>MAHHHHHHMSMFNIVRKEFQFGQHQVVLETGRVARQANTVLITMGGVTVLVAVVAAPTAKAGQDFFPLTVNYQEKQYAAGRIPGGYGKREGRASEAETLISRLIDRPIRPLFPEGYYNEIQVTATVVSSDKTMEADIAAMLGTSAALAIAGTPFRGPIGAARVGLINGEYVLNPNFEQMAQSDLDLVVAGTESAVLMVESEAKELSEDQMLGAVLFGHDEMQIAIQAINEFAAAAGAKPSDWVAPAHNEELRAKLKEAFEAKISEAYTIAVKQDRYAALDALHAEAVAQFVPEEDVDGIADEVDYLFEDLKYRTVRDNILSGKPRIDGRDTKTVRALDVQVGVLERAHGSALFTRGETQALVTTTLGNTRDALMVDTLAGTKTDNFMLHYNFPAYSVGETGRE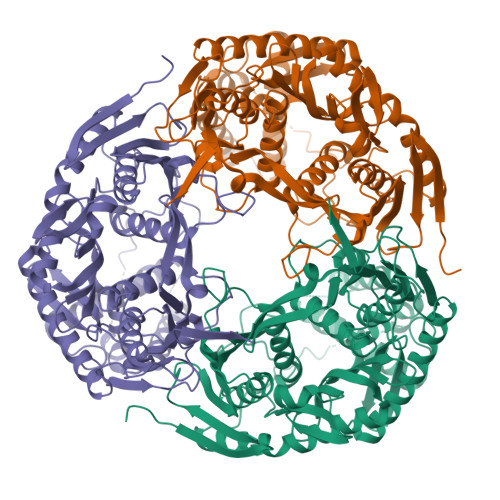SGPKRREIGHGRLARRGVQAVLPAADRFPYVIRIVSDITESNGSSSMASVCGASLSLMDAGVPLKAPVAGIAMGLVKEGERFAVLSDILGDEDHLGDMDFKVAGSANGITALQMDIKIEGITEEIMEVALNQAFAGRMHILNEMNKVISRARPEISMHAPTFEVITINPDKIRDVIGKGGATIRQITEETKAAIDIEDNGTVRVFGETKAAAKAAIAKIQAITAEVEPGKIYDGKVIRIVEFGAFVNIMPGTDGLLHISQISNERIANVTDVLKEGQEVKVQVQDVDNRGRIKLTMKDIEQA[2x]> AKMAFTLADRVTEEMLADKAALVVEVVEENYHAAPIVGIAVVNEHGRFFLRPETALADPQFVAWLGDETKKKSMFDSKRAAVALKWKGIELCGVSFDLLLAAYLLDPAQGVDDVAAAAKMKQYEAVRPDEAVYGKGAKRAVPDEPVLAEHLVRKAAAIWELERPFLDELRRNEQDRLLVELEQPLSSILAEMEFAGVKVDTKRLEQMGKELAEQLGTVEQRIYELAGQEFNINSPKQLGVILFEKLQLPVLKKTKTGYSTSADVLEKLAPYHEIVENILHYRQLGKLQSTYIEGLLKVVRPDTKKVHTIFNQALTQTGRLSSTEPNLQNIPIRLEEGRKIRQAFVPSESDWLIFAADYSQIELRVLAHIAEDDNLMEAFRRDLDIHTKTAMDIFQVSEDEVTPNMRRQAKAVNFGIVSGISDYGLAQNLNISRKEAAEFIERYFESFPGVKRYMENIVQEAKQKGYVTTLLHRRRYLPDITSRNFNVRSFAERMAMNTPIQGSAADIIKKAMIDLNARLKEERLQAHLLLQVHDELILEAPKEE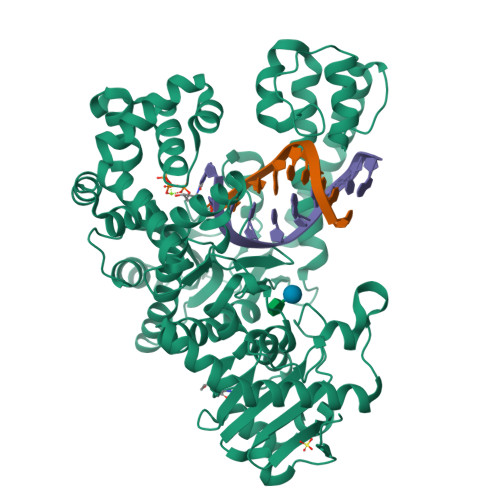MERLCRLVPEVMEQAVTLRVPLKVDYHYGSTWYDAK> 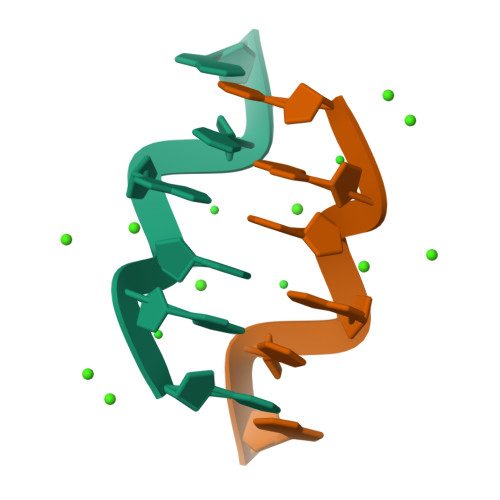CGCGCG>[2x]GPAPA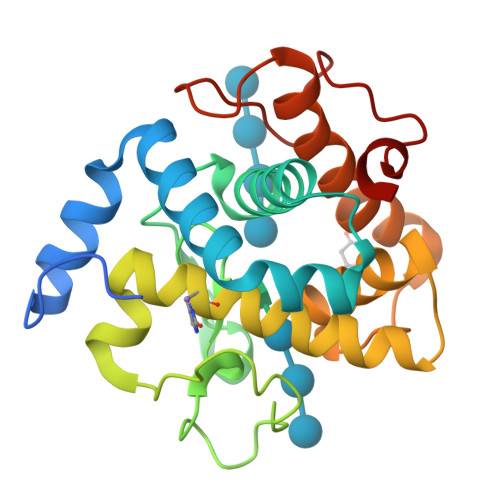NTQSGILNDGYFPPGTSKHELIARASSLKVSEVKAIIKKQVDEHWDVIRDVCGFKNKEVAYAFFFGMATRESTFRAATETGSGASHAFGPLQTAETAYANANPNYMPEHNVPEMHQYDFTEYNFYDVGISVHMGIRHFLHFARLAKEKYSGRDIARHGLMGYNTGWIDGADESWIVRYADETAALGAWYLRNNHMSDDEFTWDTDPRVDRSNPWEIYY>[4x]VLGGHECQPHSQPWQA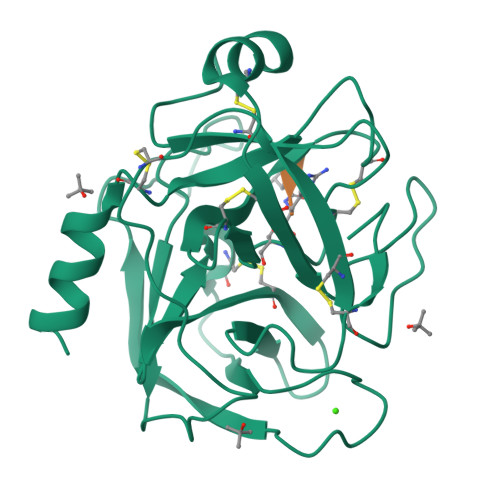ALFQGQQLLCGGVLVGGNWVLTAAHCKKPKYTVRLGDHSLQNKDGPEQEIPVVQSIPHPCYNSSDVEDHNHDLMLLQLRDQASLGSKVKPISLADHCTQPGQKCTVSGWGTVTSPRENFPDTLNCAEVKIFPQKKCEDAYPGQITDGMVCAGSSKGADTCQGDSGGPLVCDGALQGITSWGSDPCGRSDKPGVYTNICRYLDWIKKIIGSKG> GFPCGESCVYLPCFTAAIGCSCKSKVCY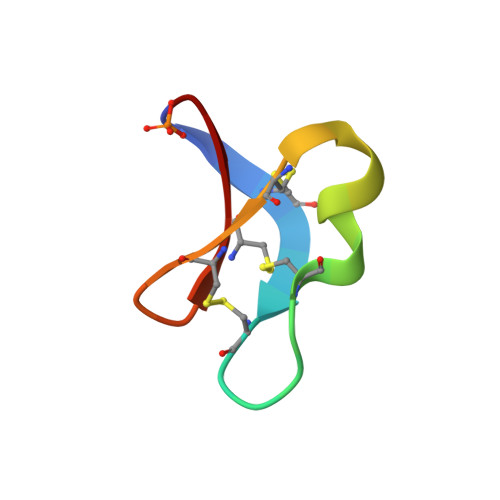KN>[3x]MSDLVRVERKGRVTTVILNRPASRNAVNGPTAAALCAAFEQFDRDDAASVAVLWGAGGTFCAGADLKAFGTPEANSVHRTGPGPMGPSRMMLSKPVIAAVSGYAVAGGLELALWCDLRVAEEDAVFGVFCRRWGVPLIDGGTVRLPRLIGHSRAMDMILTGRGVPADEALAMGLANRVVPKGQARQAAEELAAQLAALPQQCLRSDRLSALHQWGLPESAALDLEF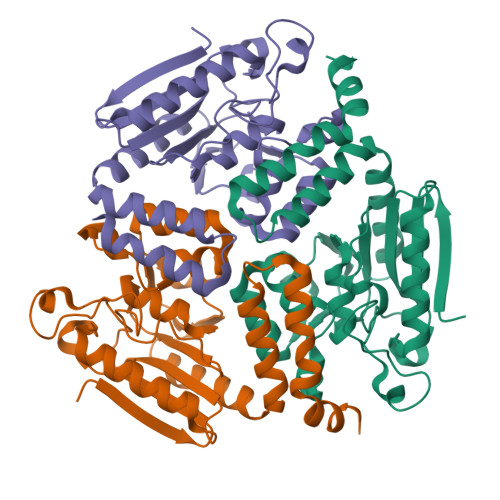ASIARVAGEALEGARRFAAGAGRHGAPAPRAEQGDTLHHHHHH> MDKDEAWKCVEQLRREGATQIAYRSDDW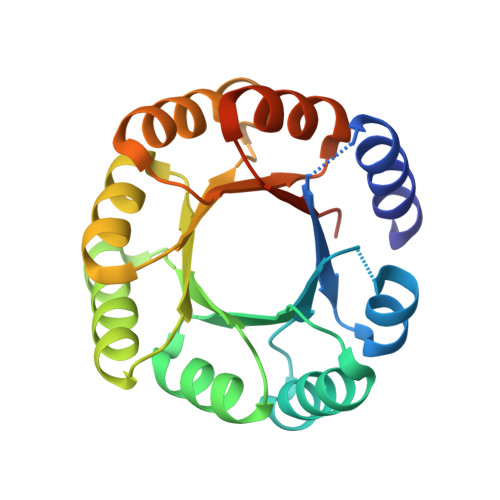RDLKEAWKKGADILIVDATDKDEAWKQVEQLRREGATQIAYRSDDWRDLKEAWKKGADILIVDATDKDEAWKQVEQLRREGATQIAYRSDDWRDLKEAWKKGADILIVDATDKDEAWKQVEQLRREGATQIAYRSDDWRDLKEAWKKGADILICDATGLEHHHHHH> GDADVLVKWSEDLANLPSIDTQHKRLVDYINDLYRAARRRDMDKAREVFDALKNYAVEHFGYEERLFADYAYPEATRHKEIHRRFVETVLKWE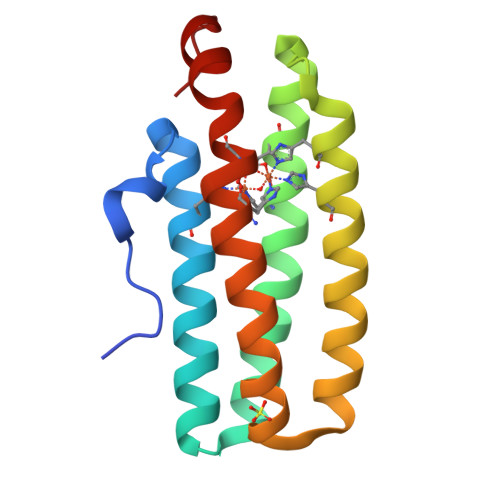KQLAAGDPEVVMTTLRGLVDWLVNHIMKEDKKYEAYLRERGVS>GGSHMKSYEIALIGNPNVGKSTIFNALTGENVYIGNWPGVTVEKKEGEFEYNGEKFKVVDLPGVYSLTANSIDEIIARDYIINEKPDLVVNIVDATALERNLYLTLQLMEMGANLLLALNKMDLAKSLGIEIDVDKLEKILGVKVVPLSAAKKMGIEELKKAISIAVKDKKTAEIKYPNFEPYIKKIT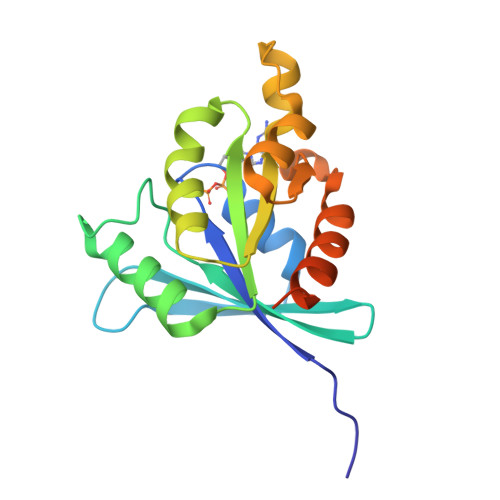[2x];> AAAAAAA>[2x]KESAAAKFERQHMDSGNSASSSSNYCNLMMCCRKMTQGKCKPVNTFVHESLADVKAV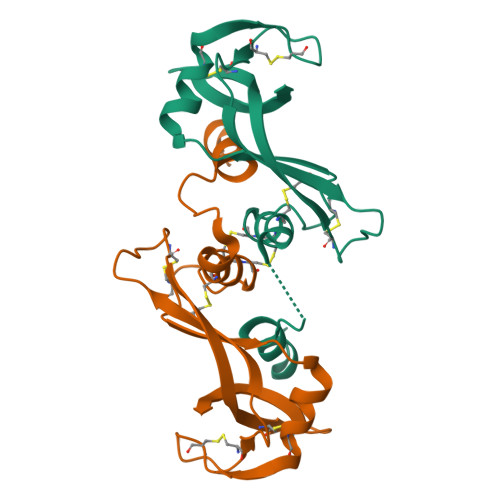CSQKKVTCKDGQTNCYQSKSTMRITDCRETGSSKYPNCAYKTTQVEKHIIVACGGKPSVPVHFDASV3-PYRROLIDIN-1-YL-N-[6-(3-PYRROLIDIN-1-YL-PROPIONYLAMINO)-ACRIDIN-3-YL]-PROPIONAMIDE | C27 H33 N5 O2 | 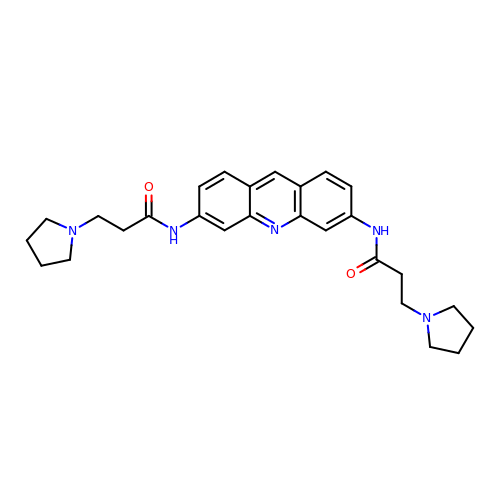WQSTTZVZUNIDBE-UHFFFAOYSA-N>[2x]MSLTNHEQVLTDYLAAFIEELVQAGVKEAIISPGSRSTPLALMMAEHPILKIYVDVDERSAGFFALGLAKASKRPVVLLCTSGTAA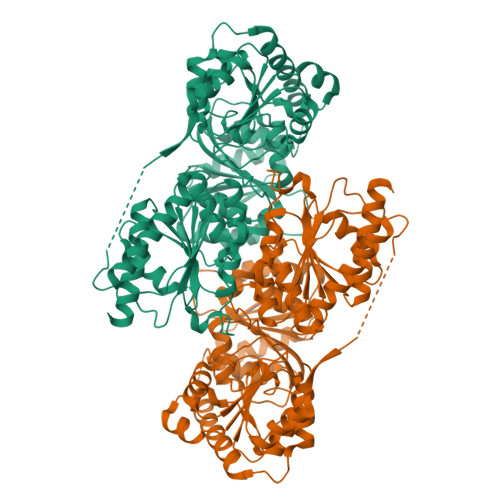ANYFPAVAEANLSQIPLIVLTADRPHELRNVGAPQAMDQLHLYGSHVKDFTDMALPENSEEMLRYAKWHGSRAVDIAMKTPRGPVHLNFPLREPLVPILEPSPFTATGKKHHHVHIYYTHEVLDDSSIQKMVTECTGKKGVFVVGPIDKKELEQPMVDLAKKLGWPILADPLSGLRSYGALDEVVIDQYDAFLKEAEIIDKLTPEVVIRFGSMPVSKPLKNWLEQLSDIRFYVVDPGAAWKDPIKAVTDMIHCDERFLLDIMQQNMPDDAKDAAWLNGWTSYNKVAREIVLAEMANTTILEEGKIVAELRRLLPDKAGLFIGNSMPIRDVDTYFSQIDKKIKMLANRGANGIDGVVSSALGASVVFQPMFLLIGDLSFYHDMNGLLMAKKYKMNLTIVIVNNDGGGIFSFLPQANEPKYFESLFGTSTELDFRFAAAFYDADYHEAKSVDELEEAIDKASYHKGLDIIEVKTNRHENKANHQALEGHHHHHH>GPLGSKASNNDDHNYVYPLPENMVYRFNKSTNILDYLSTERDHVMMAVQYYMSKQRLDDLYRQLPTKTRSYIDIINMYCDKVNNDYNRDMNIMYDMASTESFTVYDINNEVNTILMDNKGLGVRLATISFITELGKRCMNPVETIKMFTLLSHTICDDCFIDYITDIS[6x];>PSSTMGQVGRQLAIIGDDINRRYDSE[6x]

Variola virus (VAR), the causative agent of smallpox, is a member of the poxvirus family and belongs to the orthopoxviridae. The B-cell lymphoma 2 (Bcl-2) protein family is a key mediator for maintaining cell survival or to drive apoptosis, thereby removing infected, damaged or unwanted cells, and sequence, structural and functional orthologs of Bcl-2 have been found in a number of poxviruses. Here we report that despite possessing a nearly identical 3D structure and sequence, VAR F1L inhibits apoptosis via a different mechanism compared with its homolog in VV. As observed previously for VV F1L,22, 23 VAR F1L adopts a Bcl-2-like fold that forms a domain-swapped Bcl-2 with similar binding grooves that engage BH3-domain ligands.

To investigate the molecular basis for Bid, Bak and Bax BH3 domain binding by VAR F1L, we determined crystal structures of VAR F1L in complex with Bak and Bid BH3 domain peptides. Similarly, VAR F1L bound Bax and Bak BH3 domains weakly with KD values of 920 and 2640 nM, respectively. In the VAR F1L:Bak BH3 complex, residues V75, L78, I81, I85 protrude into four pockets in the VAR F1L-binding groove, similar to the equivalent hydrophobic residues in Bid (I86, L90, V93, M97). Superimposition of bound Bak and Bid BH3 backbones indicate that both ligands are bound in near identical manner. Superimposition of VV F1L with VAR F1L from their respective complexes with Bak BH3 yields a root-mean-square deviation of 0.9 Å over 138 Cα atoms, with the only notable differences in side chain orientations between VV F1L and VAR F1L occurring at F135. Overall, the VV F1L and VAR_F1L complexes with Bak appear to be near identical. Similar to endogenous mammalian pro-survival Bcl-2, VAR F1L is able to prevent both Bak- and Bax-induced yeast death, indicating that VAR F1L is able to directly engage both Bak and Bax. Unexpectedly, VAR F1L was unable to protect both wild-type and Bax−/− mouse embryonic fibroblasts (MEFs), whereas Bak−/− MEFs were efficiently protected from apoptosis in a manner similar to Bcl-2, suggesting that VAR F1L exclusively inhibits Bax-mediated apoptosis. Overall, the cellular assays mirror our peptide-binding data obtained by ITC, where the lower affinity ligand Bak is not inhibited in a cellular context. Among the other alternatively proposed mechanisms invoked to control apoptosis, VAR F1L's ability to inhibit apoptosis is most readily explained by an indirect model based on sequestration of Bax and Bak,39, 40 where Bax and Bak are held in an inactive configuration by a pro-survival Bcl-2 family member. This is supported by our observations that VAR F1L is able to bind BH3 domain peptides from Bax and Bak, albeit at modest affinity, as well as the prevention of Bax- and Bak-induced growth arrest in yeast-based assays in the absence of any other cellular apoptosis regulatory proteins.>ANPCCSNPCQNRGECMSTGFDQYKCDCTRTGFYGENCTTPEFLTRIKLLLKPTPNTVWYILTHFKGVWNIVNNIPFLRSLIMKYVLTSRSYLIDSPPTYNVHYGYKSWEAFSNLSYYTRALPPVADDCPTPMGVKGNKELPDSKEVLEKVLLRREFIPDPQGSNMMFAFFAQHFTHQFFKTDHKRGPGFTRGLGHGVDLNHIYGETLDRQHKLRLFKDGKLKYQVIGGEVYPPTVKDTQVEMIYPPHIPENLQFAVGQEVFGLVPGLMMYATIWLREHNRVCDILKQEHPEWGDEQLFQTSRLILIGETIKIVIEDYVQHLSGYHFKLKFDPELLFNQQFQYQNR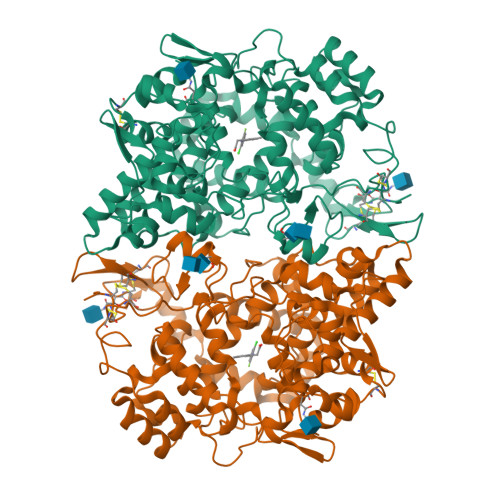IASEFNTLYHWHPLLPDTFNIEDQEYSFKQFLYNNSILLEHGLTQFVESFTRQIAGRVAGGRNVPIAVQAVAKASIDQSREMKYQSLNEYRKRFSLKPYTSFEELTGEKEMAAELKALYSDIDVMELYPALLVEKPRPDAIFGETMVELGAPFSLKGLMGNPICSPQYWKPSTFGGEVGFKIINTASIQSLICNNVKGCPFTSFNVQDPQPTKTATINASASHSRLDDINPTVLIKRRSTEL[4x]> MDYKDDDDKGDHNHRHKHGDPHMSEKRSLPMVDVKIDDEDTPQLEKKIKRQSIDHGVGSEPVSTIEIIPSDSFRKYNSQGFKAKDTDLMGTQLESTFEQELSQMEHDMADQEEHDLSSFERKKLPTDFDPSLYDISFQQIDAEQSVLNGIKDENTSTVVRFFGVTSEGHSVLCNVTGFKNYLYVPAPNSSDANDQEQINKFVHYLNETFDHAIDSIEVVSKQSIWGYSGDTKLPFWKIYVTYPHMVNKLRTAFERGHLSFNSWFSNGTTTYDNIAYTLRLMVDCGIVGMSWITLPKGKYSMIEPNNRVSSCQLEVSINYRNLIAHPAEGDWSHTAPLRIMSFDIECAGRIGVFPEPEYDPVIQIANVVSIAGAKKPFIRNVFTLNTCSPITGSMIFSHATEEEMLSNWRNFIIKVDPDVIIGYNTTNFDIPYLLNRAKALKVNDFPYFGRLKTVKQEIKESVFSSKAYGTRETKNVNIDGRLQLDLLQFIQREYKLRSYTLNAVSAHFLGEQKEDVHYSIISDLQNGDSETRRRLAVYCLKDAYLPLRLMEKLMALVNYTEMARVTGVPFSYLLARGQQIKVVSQLFRKCLEIDTVIPNMQSQASDDQYEGATVIEPIRGYYDVPIATLDFNSLYPSIMMAHNLCYTTLCNKATVERLNLKIDEDYVITPNGDYFVTTKRRRGILPIILDELISARKRAKKDLRDEKDPFKRDVLNGRQLALKISANSVYGFTGATVGKLPCLAISSSVTAYGRTMILKTKTAVQEKYCIKNGYKHDAVVVYGDTDSVMVKFGTTDLKEAMDLGTEAAKYVSTLFKHPINLEFEKAYFPYLLINKKRYAGLFWTNPDKFDKLDQKGLASVRRDSCSLVSIVMNKVLKKILIERNVDGALAFVRETINDILHNRVDISKLIISKTLAPNYTNPQPHAVLAERMKRREGVGPNVGDRVDYVIIGGNDKLYNRAEDPLFVLENNIQVDSRYYLTNQLQNPIISIVAPIIGDKQANGMFVVKSIKINTGSQKGGLMSFIKKVEACKSCKGPLRKGEGPLCSNCLARSGELYIKALYDVRDLEEKYSRLWTQCQRCAGNLHSEVLCSNKNCDIFYMRVKVKKELQEKVEQLSKW;> GPGGDLHMDALLTKFNEDRSLQDENLSQPRTRVRIVDDNLYNKSNPFQLCYKKRDYGSQYYHIYQYRLKTFRERVLKECDKRWDAGFTLNGQLVLKKDKVLDIQGNQPCWCVGSIYCEMKYKPNVLDEVINDTYGAPDLTKSYTDKEGGSDEIMLEDESGRVLLVGDFIRSTPFITGVVVGILGMEAEAGTFQVLDICYPTPLPQNPFPAPIATCPTRGKIALVSGLNLNNTSPDRLLRLEILREFLMGRINNKIDDISLIGRLLICGNSVDFDIKSVNKDELMISLTEFSKFLHNILPSISVDIMPGTNDPSDKSLPQQPFHKSLFDKSLESYFNGSNKEILNLVTNPYEFSYNGVDVLAVSGKNINDICKYVIPSNDNGESENKVEEGESNDFKDDIEHRLDLMECTMKWQNIAPTAPDTLWCYPYTDKDPFVLDKWPHVYIVANQPYFGTRVVEIGGKNIKIISVPEFSSTGMIILLDLETLEAETVKIDI;> MDQKASYFINEKLFTEVKPVLFTDLIHHLKIGPSMAKKLMFDYYKQTTNAKYNCVVIC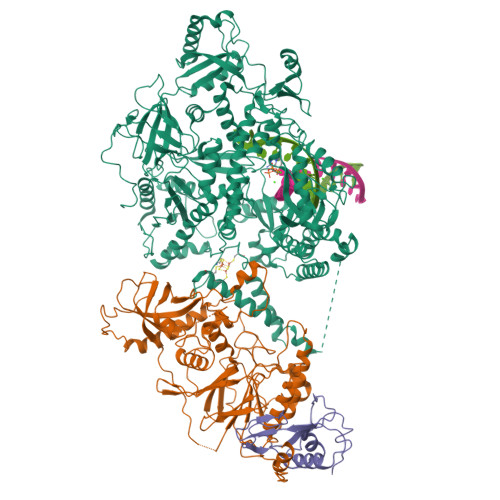CYKDQTIKIIHDLSNIPQQDSIIDCFIYAFNPMDSFIPYYDIIDQKDCLTIKNSYELKVSESSKIIERTKTLEEKSKPLVRPTARSKTTPEETTGRKSKSKDMGLRSTALLAKMKKDRDDKETSRQNELRKRKEENLQKINKQNPEREAQMKELNNLFVEDDLDTEEVNGGSKPNSPKETDSNDKDKNNDDLEDLLETTAEDSLMDVPKIQQTKPSETEHSKEPKSEEEPSSFIDEDGYIVTKRPATSTPPRKPSPVVKRALSSSKKQETPSSNKRLKKQGTLESFFKRKAK>MKEENVGDFTLHYGVFEEVEPEELRNLADMLRQRTKKDVVFIASRKGDKINFVIGVSKEISDKVNAKEVIREVGKVLKGGGGGRADLAQGGGKAPD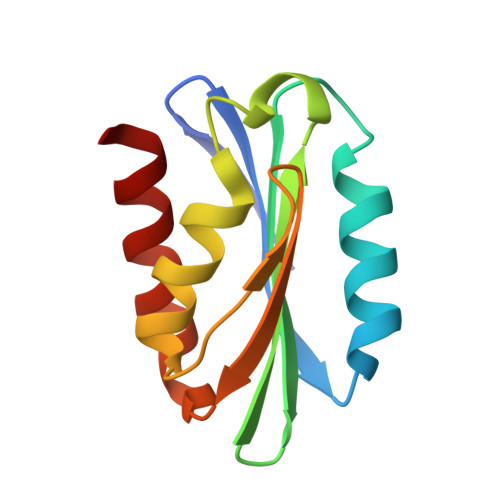KFPEAVKLLKEILSG[2x]> MRSVTNAFGNSGELNDQVDETGYRKFDIHEGILFCIELSETMFKESSDLEYKSPLLEILESLDELMSQLVITRPGTAIGCYFYYCNREDAKEGIYELFPLRDINATFMKKLNDLLEDLSSGRISLYDYFMFQQTGSEKQVRLSVLFTFMLDTFLEEIPGQKQLSNKRVFLFTDIDKPQEAQDIDERARLRRLTIDLFDNKVNFATFFIGYADKPFDNEFYSDILQLGSHTNENTGLDSEFDGPSTKPIDAKYIKSRILRKKEVKRIMFQCPLILDEKTNFIVGVKGYTMYTHEKAGVRYKLVYEHEDIRQEAYSKRKFLNPITGEDVTGKTVKVYPYGDLDINLSDSQDQIVMEAYTQKDAFLKIIGFRSSSKSIHYFNNIDKSSFIVPDEAKYEGSIRTLASLLKILRKKDKIAILWGKLKSNSHPSLYTLSPSSVKDYNEGFYLYRVPFLDEIRKFPSLLSYDDGSEHKLDYDNMKKVTQSIMGYFNLRDGYNPSDFKNPLLQKHYKVLHDYLLQIETTFDENETPNTKKDRMM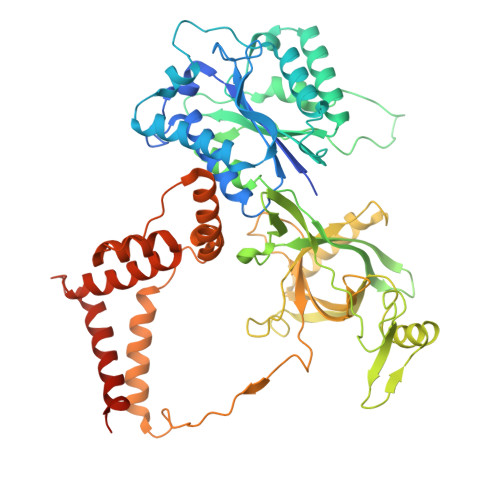REDDSLRKLYYIRNKILESEKSEDPIIQRLNKYVKIWNMFYKKFNDDNISIKEEKKPFDKKPKFNI> ATSDDWKSKAIYQLLTDRFGRADDSTSNCSNLSNYCGGTYEGITKHLDYISGMGFDAIWISPIPKNSDGGYHGYWATDFYQLNSNFGDESQLKALIQAAHERDMYVMLDVVANHAGPTSNGYSGYTFGDASLYHPKCTIDYNDQTSIEQCWVADELPDIDTENSDNVAILNDIVSGWVGNYSFDGIRIDTVKHIRKDFWTGYAEAAGVFATGEVFNGDPAYVGPYQKYLPSLINYPMYYALNDVFVSKSKGFSRISEMLGSNRNAFEDTSVLTTFVDNHDNPRFLNSQSDKALFKNALTYVLLGEGIPIVYYGSEQGFSGGADPANREVLWTTNYDTSSDLYQFIKTVNSVRMKSNKAVYMDIYVGDNAYAFKHGDALVVLNNYGSGSTNQVSFSVSGKFDSGASLMDIVSNITTTVSSDGTVTFNLKDGLPAIFTSA;> ATSDDWKSKAIYQLLTDRFGRADDSTSNCSNLSNYCGGTYEGITKHLDYISGMGFDAIWISPIPKNSDGGYHGYWATDFYQLNSNFGDESQLKALIQAAHERDMYVMLDVVANHAGPTSDGYSGYTFGDASLYHPKCTIDYNDQTSIEQCWVADELPDIDTENSDNVAILNDIVSGWVGNYSFDGIRIDTVKHIRKDFWTGYAEAAGVFATGEVFNGDPAYVGPYQKYLPSLINYPMYYALNDVFVSKSKGFSRISEMLGSNRNAFEDTSVLTTFVDNHDNPRFLNSQSDKALFKNALTYVLLGEGIPIVYYGSEQGFSGGADPANREVLWTTNYDTSSDLYQFIKTVNSVRMKSNKAVYMDIYVGDNAYAFKHGDALVVLNNYGSGSTNQVSFSVSGKFDSGASLMDIVSNITTTVSSDGTVTFNLKDGLPAIFTSA

Here, we describe the structure and function of three novel α-amylases from Cordyceps farinosa (CfAM), Rhizomucor pusillus (RpAM) and Thamnidium elegans (TeAM) with a higher stability and pH-tolerance with the potential to act as novel biocatalysts for various industrial processes. The sequence of all three enzymes groups them in the GH13 sub-family 1 along with, for example, the amylase from Aspergillus oryzae (also known as TAKA amylase). All three amylases have the classical domain structure with a central (β/α)8-barrel with the active site located on its C-terminal face, together with a small subdomain, inserted between the third strand and helix and a C-terminal β-sandwich. All three amylases have as their hallmark a shortened loop between β2/α3 and two shorter loops in subdomain B located between β3 and α4 of the central (β/α)8-barrel, compared to structures of other fungal amylases, e.g., TAKA-amylase.

The final model of RpAM includes two monomers in the asymmetric unit comprising residues 1 to 438 in both chains, which superpose on each other with an r.m.s.d. of 0.54 Å. The temperature profiles reveal that RpAM and CfAM also have a considerably higher thermotolerance compared to TAKA and TeAM. In particular, RpAM retains full activity even at 80 °C, making it an attractive enzyme for industrial high temperature starch saccharification processes. Further analysis of the sequence showed that both RpAM and CfAM have a slightly lower number of charged residues and a higher number of hydrophobic residues compared to TeAm and TAKA amylase, which might contribute to the higher thermostability of these two variants. Although all three amylases were co-crystallized with acarbose, a well-known inhibitor for amylases, a complex with acarbose bound was only obtained for TeAM and CfAM. The reason why acarbose was not bound to RpAM is not clear. There are three N-glycosylation sites, one at N144 in RpAM and two at N180 and 412 in TeAM. Indeed, N144 is located in an extended loop and N-glycosylation might help to shield the loop against proteolytic attack. We observed the formation of an isoaspartate by succinimide formation and deamidation of N120 in chain B of RpAM. The same asparagine in chain A shows high flexibility and the resulting density suggest partial isoaspartate formation, but a model could not be built with confidence.>GPMKTEMKDDFAKLEEQFDAKLGIFALDTGTNRTVAYRPDERFAFASTIKALTVGVLLQQKSIEDLNQRI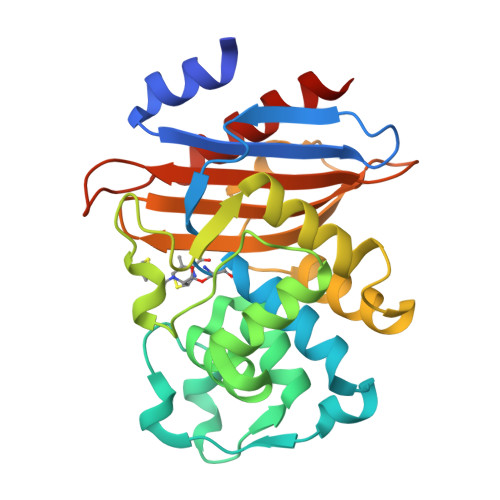TYTRDDLVNYNPITEKHVDTGMTLKELADASLRYSDNAAQNLILKQIGGPESLKKELRKIGDEVTNPERFHPELNEVNPGETQDTSTARALVTSLRAFALEDKLPSEKRELLIDWMKRNTTGDALIRAGVPDGWEVADKTGAASYGTRNDIAIIWPPKGDPVVLAVLSSRDKKDAKYDDKLIAEATKVVMKALNMNGK[2x]>QFTERALTILTLAQKLASDHQHPQLQPIHILAAFIETPEDGSVPYLQNLIEKGRYDYDLFKKVVNRNLVRIPQQQPAPAEITPSYALGKVLQDAAKIQKQQKDSFIAQDHILFALFNDSSIQQIFKEAQVDIEAIKQQALELRGNTRIDSRGADTNTPLEYLSKYAIDMTEQARQGKLDPVIGREEEIRSTIRVLARRIKSNP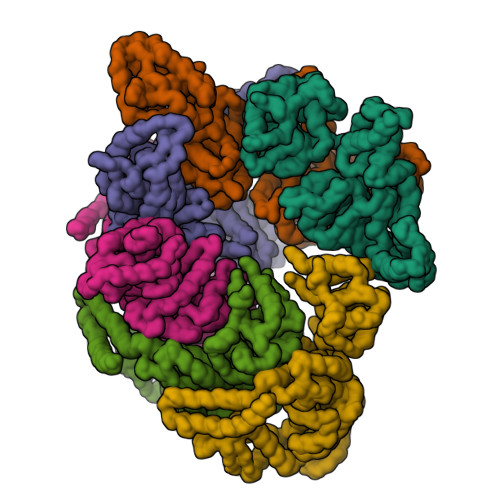CLIGEPGIGKTAIIEGVAQRIIDDDVPTILQGAKLFSLDLAALTAGAKYKGDFEERFKGVLKEIEESKTLIVLFIDEIHMLMGNGKDDAANILKPALSRGQLKVIGATTNNEYRSIVEKDGAFERRFQKIEVAEPSVRQTVAILRGLQPKYEIHHGVRILDSALVTAAQLAKRYLPYRRLPDSALDLVDISCAGVAVARDSKPEELDSKERQLQLIQVEIKALERDEDADSTTKDRLKLARQKEASLQEELEPLRQRYNEEKHGHEELTQAKKKLDELENKALDAERRYDTATAADLRYFAIPDIKKQIEKLEDQVAEEERRAGANSMIQNVVDSDTISETAARLTGIPVKKLSESENEKLIHMERDLSSEVVGQMDAIKAVSNAVRLSRSGLANPRQPASFLFLGLSGSGKTELAKKVAGFLFNDEDMMIRVDCSELSEKYAVSKLLGTTAGYVGYDEGGFLTNQLQYKPYSVLLFDEVEKAHPDVLTVMLQMLDDGRITSGQGKTIDCSNCIVIMTSNLGAEFINSQQGSKIQESTKNLVMGAVRQHFRPEFLNRISSIVIFNKLSRKAIHKIVDIRLKEIEERFEQNDKHYKLNLTQEAKDFLAKYGYSDDMGARPLNRLIQNEILNKLALRILKNEIKDKETVNV[6x]ethyl 1-(2-piperidin-4-ylethyl)-5-pyridin-4-yl-indole-2-carboxylate | C23 H27 N3 O2 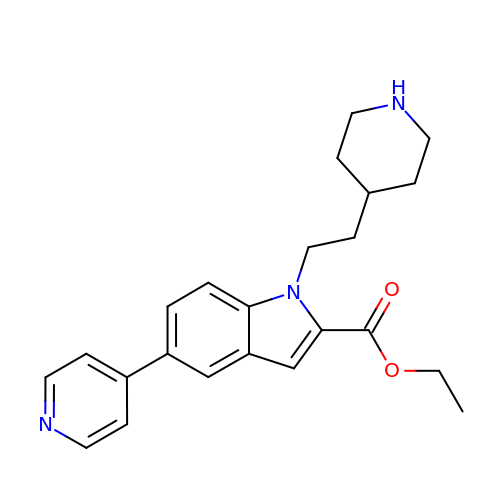| WFSAKSOITHNEMN-UHFFFAOYSA-N> GMIQVPA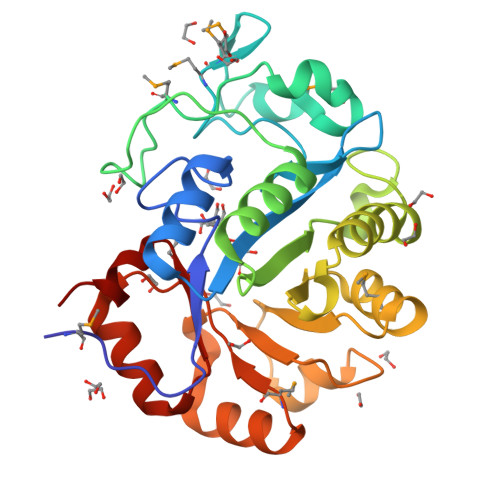SFDIQGHRGCRGLLPENTIAAFTKALLLGVTTLEFDLVISKDNRVVVSHDTFFHHEITMMVDGEDVTEANEKNFNLYAMNYADIKEIDVGMKTHPRFKSQKKVPAVKPLFRELIETAEKLSAKIQYNGEIKSTVEGDNIDHPNIALFCDLVVAEIKKAHITDRFTLQSFDVRALEYMHSQYPDIKLSYLVETKGTLKKQLEKLSFTPAVYSPDVTLVSKKDIDAAHKLGMRVIPWTVNTKEEIETLISLGVDGIITDYPDLFFEK> HHHHHHMPSYKSSRVLVRDVPEELVDHYERSHRVAAFFMRLLLAMRREPYSLRMRDGTEREVDLDETDDFLRSAGCEEPDAVSDDLRSFALAVLHQDNPKKRAFLESENCVSILCLEKSASGTRYYKRPGYQLLKKAIEEEWGWDKFEASLLDERTGEVAEKFAALSMEDWRRFFAARDPDDLGRELLKTDTREGMAAALRLRERGVFPVSVPEHLDLDSLKAAMASAAERLKSWLACNQRAVDEKSELRKRFEEALDGVDPEKYALFEKFAAELQQADYNVTKKLVLAVSAKFPATEPSEFKRGVEILKEDGYKPLWEDFRELGFVYLAERKWERRRGGAAVTLCDADDSPIKVRFGLTGRGRKFVLSAAGSRFLITVKLPCGDVGLTAVPSRYFWNPSVGRTTSNSFRIEFTKRTTENRRYVGEVKEIGLVRQRGRYYFFIDYNFDPE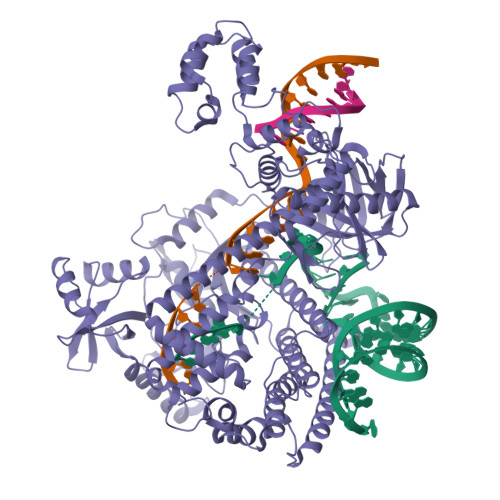EVSDETKVGRAFFRAPLNESRPKPKDKLTVMGIDLGINPAFAFAVCTLGECQDGIRSPVAKMEDVSFDSTGLRGGIGSQKLHREMHNLSDRCFYGARYIRLSKKLRDRGALNDIEARLLEEKYIPGFRIVHIEDADERRRTVGRTVKEIKQEYKRIRHQFYLRYHTSKRDRTELISAEYFRMLFLVKNLRNLLKSWNRYHWTTGDRERRGGNPDELKSYVRYYNNLRMDTLKKLTCAIVRTAKEHGATLVAMENIQRVDRDDEVKRRKENSLLSLWAPGMVLERVEQELKNEGILAWEVDPRHTSQTSCITDEFGYRSLVAKDTFYFEQDRKIHRIDADVNAAINIARRFLTRYRSLTQLWASLLDDGRYLVNVTRQHERAYLELQTGAPAATLNPTAEASYELVGLSPEEEELAQTRIKRKKREPFYRHEGVWLTREKHREQVHELRNQVLALGNAKIPEIRT> GSHMSQTEPPEDLMQYEAMAQDALRGVVKAALKKAAAPGGLPEPHHLYITFKTKAAGVSGPQDLLSKYPDEMTIVLQHQYWDLAPGETFFSVTLKFGGQPKRLSVPYAA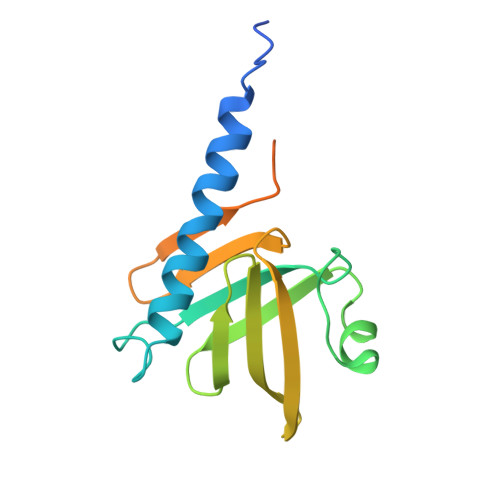LTRFYDPSVQFALQFSAPEIIEDEPEPDPEPEDKANQGASGDEGPKIV> SVDMALGDLMVSRFSQSSVSLVSNHRYDEDCVSSHDDGDSRRKDSEAKSSSSYGNGTTEGAATATSMAYLPQTIVLCELRHDASEASAPLGTSEIVLVPKWRLKERMKTGCVALVLCLNITVDPPDVIKISPCARIEAWIDPFSMAPPKALETIGKNLSTQYERWQPRARYKVQLDPTVDEVRKLCLTCRKYAKTERVLFHYNGHGVPKPTANGEIWVFNKSYTQYIPLPISELDSWLKTPSIYVFDCSAARMILNAFAELHDWGSSGSSGSSRDCILLAACDVHETLPQSVEFPADVFTSCLTTPIKMALKWFCRRSLLKEIIDESLIDRIPGRQNDRKTLLGELNWIFTAVTDTIAWNVLPHELFQRLFRQDLLVASLFRNFLLAER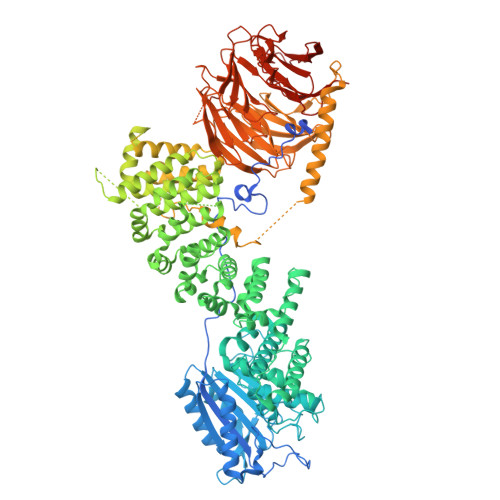IMRSANCNPISHPMLPPTHQHHMWDAWDMAAEICLSQLPQLVLDPSTEFQPSPFFTEQLTAFEVWLDHGSEHKKPPEQLPIVLQVLLSQCHRFRALVLLGRFLDMGSWAVDLALSVGIFPYVLKLLQTTTNELRQILVFIWTKILALDKSCQIDLVKDGGHTYFIRFLDSSGAFPEQRAMAAFVLAVIVDGHRRGQEACLEANLIGVCLGHLEASRPSDPQPEPLFLQWLCLCLGKLWEDFMEAQIMGREANAFEKLAPLLSEPQPEVRAAAVFALGTLLDIGFDSNKSVVEDEFDDDEKIRAEDAIIKSLLDVVSDGSPLVRAEVAVALARFAFGHKQHLKLAAASYWKPQSSSLLTSLPSIAKFHDPGSATIVSLHMSPLTRASTDSQPVARESRISSSPLGSSGLMQGSPLSDDSSLHSDSGMMHDSVSNGAVHQPRLLDNAVYSQCVRAMFALAKDPSPRIASLGRRVLSIIGIEQVVAKPSKPTGRPGEAADSGLADPLLGASGSERSLLPLSTIYGWSCGHFSKPLLGGADASQEIAAKREEKEKFALEHIAKCQHSSISKLNNNPIANWDTRFETGTKTALLHPFSPIVVAADENERIRVWNYEEATLLNGFDNHDFPDKGISKLCLINELDDSLLLVASCDGSVRIWKNYATKGKQKLVTGFSSIQGHKPGARDLNAVVDWQQQSGYLYASGETSTVTLWDLEKEQLVRSVPSESECGVTALSASQVHGGQLAAGFADGSLRLYDVRSPEPLVCATRPHQKVERVVGLSFQPGLDPAKVVSASQAGDIQFLDLRTTRDTYLTIDAHRGSLTALAVHRHAPIIASGSAKQLIKVFSLQGEQLGIIRYYPSFMAQKIGSVSCLTFHPYQVLLAAGAADSFVSIYTHDNSQAR> MSQLTEFISCIPVVNEEQNEEDERGLCKIQIEDGAMLETLDENSLSGLRIEKMLVSEGTGIFSKSSFGINDLRIFTGENIDEESKKYVWYELLKMLTGHKVYIASLDEKVVFTKWTCRMQDDEVWKVVMELESSAIIRKIAE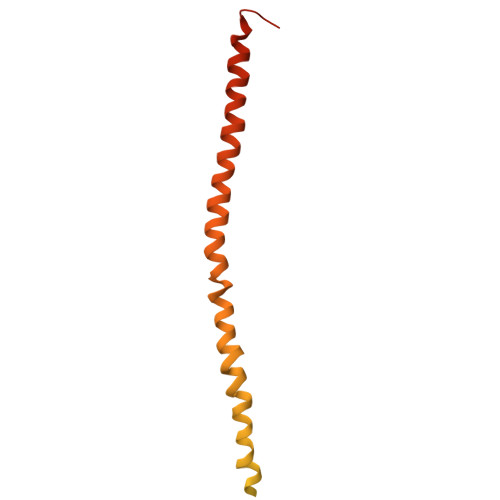LTLHPVKKGEIDLFEMADKLYKDICCVNDSYRNIKESDSSNRNRVEQLARERELLDKLLETRDERTRAMMVTLLNEKKKKIRELHEILRQNNIKLSDDDVLDSA>MDEDGNLQISNSNYNGEEEGEDPENNTLNQPLLKRHRTLSSTPLALVGAKVSHIESLDYEINENDLFKHDWRSRSKAQVFQYIFLKWTLACLVGLFTGLIATLINLAVENIAGYKLLAVGYYIAQDRFWTGLMVFTGANLGLTLVATVLVVYFAPTAAGPGIPEIKAYLNGIDTPNMFGFTTMMVKIVGSIGAVAAGLDLGKEGPLVHIGSCIASLLGQGGPDNHRIKWRWLRYFNNDRDRRDLITCGSASGVCAAFRSPVGGVLFALEEVATWWRSALLWRTFFSTAVVVVVLRAFIEICNSGKCGLFGSGGLIMFDVSHVEVRYHAADIIPVTLIGVFGGILGSLYNHLLHKVLRLYNLINQKGKIHKVLLSLGVSLFTSVCLFGLPFLAECKPCDPSIDEICPTNGRSGNFKQFNCPNGYYNDLSTLLLTTNDDAVRNIFSSNTPNEFGMVSLWIFFGLYCILGLITFGIATPSGLFLPIILMGSAYGRMLGTAMGSYTNIDQGLYAVLGAASLMAGSMRMTVSLCVIFLELTNNLLLLPITMFVLLIAKTVGDSFNLSIYEIILHLKGLPFLEANPEPWMRNLTVGELNDAKPPVVTLNGVEKVANIVDVLRNTTHNAFPVLDGADQNTGTELHGLILRAHLVKVLKKRWFLNEKRRTEEWEVREKFTPVELAEREDNFDDVAITSSEMQLYVDLHPLTNTTPYTVVQSMSVAKALVLFRSVGLRHLLVVPKIQASGMSPVIGILTRQDLRAYNILQAFPHLDKHKSGKARASGGSLEVLFQGPGGSGGSWSHPQFEK[2x]

pmcMembers of the chloride channel (CLC) family play an important role in anion transport in bacteria, animals, and plants. AtCLCa mediates nitrate storage in plant vacuoles. ATP inhibits the transport activity of AtCLCa, while AMP prevents this inhibition by competing with ATP. CLC protein forms a homodimer in which each protomer contains its own ion transport pathway, in which three anion-binding sites were identified.

Here, we report the cryo-EM structure of ATP-bound AtCLCa, which reveals the molecular features critical for its nitrate selectivity and ATP regulation. The structure of AtCLCa was determined to a resolution of 2.8 Å, allowing confident model building of most of the protein regions. Similar to the structures of other CLC proteins, AtCLCa forms a homodimer displaying C2 symmetry. The cytoplasmic domain consists of the N-terminus and two C-terminal cystathionine ß-synthase domains (CBS1 and CBS2). The side chain of Glugate (Glu203) adopts the ‘up’ conformation, pointing toward the luminal side. Three nonprotein densities can be identified in the map with intensities of ∼15 σ, ∼13 σ, and ∼12 σ, corresponding to ions bound at the external, central, and internal binding sites, respectively. In AtCLCa, nitrate is similarly coordinated by the side chain of Tyr564 and backbone nitrogen atoms from the N-terminal end of helix αN, but a hydrogen bond cannot be formed between the anion and the side chain of Pro160, which likely explains the weakened chloride preference. Additionally, the side chains of Phe471, Phe480, and Tyr564 around the central binding site exhibit noticeable outward shifts relative to the anion, which seems to be structural rearrangement to accommodate the larger nitrate. Mg2+-bound endogenous ATP can be modeled in a large nonprotein density located at the interface of the N-terminus and the two CBS domains. The γ-phosphate forms hydrogen bonds with the side chains of Ser56 in the N-terminus and Arg729 of CBS2, which further forms a salt bridge with Asp58 in the N-terminus.>[2x]MSCYIYWDKIKRIASRLEGMNYHFDEMDTSGVMPLLDEIEEIAHDSTIDFESAKHILDDAEMNHALSLIRKFYVNLGMKLQMEKAQEVIESDSPWETLRSFYFYPRYLELLKNEAALGRFRRGERAVFIGGGPLPLTGI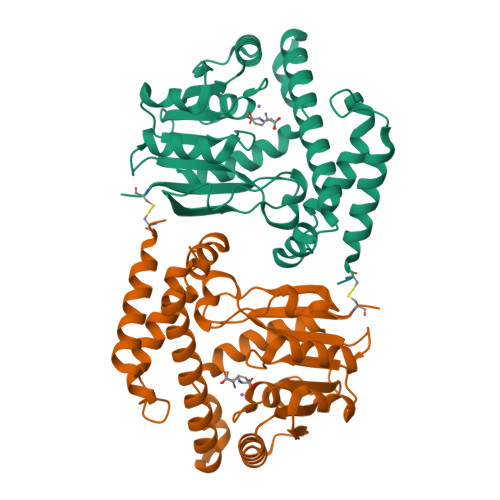LLSHVYGMRVNVVEIEPDIAELSRKVIEGLGVDGVNVITGDETVIDGLEFDVLMVAALAEPKRRVFRNIHRYVDTETRIIYRTYTGMRAILYAPVSDDDITGFRRAGVVLPSGKVNNTSVLVFKCPDKGELNSKLEGKPIPNPLLGLDSTRTGHHHHHH> MTTTESPTAAGSGSAATDKFKAERATADTSPERLAAIAKDALGALN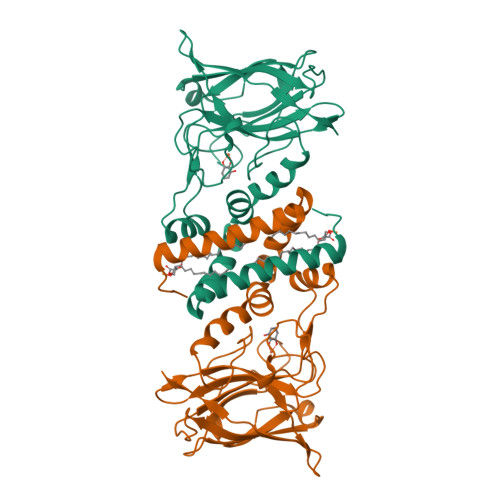DVILKHGVTYPEYRVFKQWLIDVGEGGEWPLFLDVFIEHSVEEVLARSRKGTMGSIEGPYYIENSPELPSKCTLPMREEDEKITPLVFSGQVTDLDGNGLAGAKVELWHADNDGYYSQFAPHLPEWNLRGTIIADEEGRYEITTIQPAPYQIPTDGPTGQFIEAQNGHPWRPAHLHLIVSAPGKESVTTQLYFKGGEWIDSDVASATKPELILDPKTGDDGKNYVTYNFVLDPA The PI3K-related kinase (PIKK) SMG1 monitors the progression of metazoan nonsense-mediated mRNA decay (NMD) by phosphorylating the RNA helicase UPF1. SMG1 is a member of the phosphatidylinositol-3-kinase-related kinase (PIKK) family, which also includes the ATM, ATR, DNA-PKc, and mTOR kinases. Despite the confounding name reflecting a possible evolutionary origin with a lipid kinase, and in retrospect the ability of some PIKK family members to bind inositol-6-phosphate, all active PIKKs are Ser-Thr protein kinases. These large, multidomain enzymes share an overall similar architecture: a C-terminal catalytic module (comprising the so-called FAT, kinase, and FATC domains) and an N-terminal α-solenoid (that typically serves as a protein-protein interaction module). SMG8 and SMG9 form an unusual G-domain heterodimer.

In this manuscript, we reported a reconstruction of the SMG1-8-9 complex bound to an SMG1 inhibitor. We showed that this compound binds to the ATP-binding site within the kinase active site. While many of the SMG1 residues interacting with SMG1i are conserved within the PIKK family, two contact sites appear to be specific: SMG1 Pro2213 and Asp2339 contact the sulfonamide moiety of the inhibitor while Asn2356 forms hydrogen bonds with the phenyl urea/carbamide group. Superposition of the SMG1 active site in the SMG1i-bound structure with the active site of mTORΔN shows that the corresponding residues have diverged and would not be able to mediate analogous interactions with the SMG1i sulfonamide group (mTOR Thr2245 and Ser2342 at the positions of SMG1 Pro2213 and Asp2339) or with the urea group (mTOR Gly2359 at the position of SMG1 Asn2356). Taken together, these observations rationalize the specificity of SMG1i for SMG1 over mTORΔN that we observed in the in vitro assays. Superposition with other PIKKs suggests the presence of potentially similar discriminatory interactions: like mTOR, DNA-PK lacks a favorable interaction site for the SMG1i urea group (Gly3943 at the position of SMG1 Asn2356). In the case of ATR, the SMG1i sulfonamide site has diverged (Gly2385 at the position of SMG1 Pro2213) and residues in the N-lobe would result in a steric clash with the urea group of the inhibitor (Lys2329 and Asp2330 corresponding to SMG1 Leu2157 and Glu2158). Finally, mTOR, DNA-PK, and ATR active sites have a different relative orientation of the kinase N- and C-lobes as compared to SMG1, changing the overall chemical environment at the SMG1i-binding site. We conclude that subtle differences in the SMG1 structure underpin the specificity of the SMG1i inhibitor.

> ANTLVEDVNICLQACSSLHALSSSLPDDLLQRCVDVCRVQLVHSGTRIRQAFGKLLKSIPLDVVLSNNNHTEIQEISLALRSHMSKAPSNTFHPQDFSDVISFILYGNSHRTGKDNWLERLFYSCQRLDKRDQSTIPRNLLKTDAVLWQWAIWEAAQFTVLSKLRTPLGRAQDTFQTIEGIIRSLAAHTLNPDQDVSQWTTADNDEGHGNNQLRLVLLLQYLENLEKLMYNAYEGCANALTSPPKVIRTFFYTNRQTCQDWLTRIRLSIMRVGLLAGQPAVTVRHGFDLLTEMKTTSLSQGNELEVTIMMVVEALCELHCPEAIQGIAVWSSSIVGKNLLWINSVAQQAEGRFEKASVEYQEHLCAMTGVDCCISSFDKSVLTLANAGRNSASPKHSLNGESRKTVLSKPTDSSPEVINYLGNKACECYISIADWAAVQEWQNSIHDLKKSTSSTSLNLKADFNYIKSLSSFESGKFVECTEQLELLPGENINLLAGGSKEKINMKKLLPNMLSPDPRELQKSIEVQLLRSSVCLATALNPIEQDQKWQSITENVVKYLKQTSRIAIGPLRLSTLTVSQSLPVLSTLQLYCSSALENTVSNRLSTEDCLIPLFSEALRSCKQHDVRPWMQALRYTMYQNQLLEKIKEQTVPIRSHLMELGLTAAKFARKRGNVSLATRLLAQCSEVQLGKTTTAQDLVQHFKKLSTQGQVDEKWGPELDIEKTKLLYTAGQSTHAMEMLSSCAISFCKSVKAEYAVAKSILTLAKWIQAEWKEISGQLKQVYRAQHQQNFTGLSTLSKNILTLIELPSVNTMEEEYPRIESESTVHIGVGEPDFILGQLYHLSSVQAPEVAKSWAALASWAYRWGRKVVDNASXXXXXXXXXXXXXXXXXXXXXXXXXXXXXXXXXXXXXXXXXXXXXXXXXXXXXXXXXXXXXXXXXXXXXXXXXXXXXXXXXXXXXXXXEGVIKVWRKVVDRIFSLYKLSCSAYFTFLKLNAGQIPLDEDDPRLHLSHRVEQSTDDMIVMATLRLLRLLVKHAGELRQYLEHGLETTPTAPWRGIIPQLFSRLNHPEVYVRQSICNLLCRVAQDSPHLILYPAIVGTISLSSESQASGNKFSTAIPTLLGNIQGEELLVSECEGGSPPASQDSNKDEPKSGLNEDQAMMQDCYSKIVDKLSSANPTMVLQVQMLVAELRRVTVLWDELWLGVLLQQHMYVLXXXXXXXXXXXXXXXXXXXXXXXXXXXXXXXXXXXXXXXXXXXXXXXXXXXXXXXXPHEKWFQDNYGDAIENALEKLKXXXXXXXXXXXXXXXXXXXXXXXXXXXXXXXYILRLEEISPWLAAMTNTEIALPGEVSARDTVTIHSVGGTITILPTKTKPKKLLFLGSDGKSYPYLFKGLEDLHLDERIMQFLSIVNTMFATINRQETPRFHARHYSVTPLGTRSGLIQWVDGATPLFGLYKRWQQREAALQAQKAQDSYQTPQNPGIVPRPSELYYSKIGPALKTVGLSLDVSRRDWPLHVMKAVLEELMEATPPNLLAKELWSSCTTPDEWWRVTQSYARSTAVMSMVGYIIGLGDRHLDNVLIDMTTGEVVHIDYNVCFEKGKSLRVPEKVPFRMTQNIETALGVTGVEGVFRLSCEQVLHIMRRGRETLLTLLEAFVYDPLVDWTAGGEAGFAGAVYGGGGQQAESKQSKREMEREITRSLFSSRVAEIKVNWFKNRDEMLVVLPKLDGSLDEYLSLQEQLTDVEKLQGKLLEEIEFLEGAEGVDHPSHTLQHRYSEHTQLQTQQRAVQEAIQVKLNEFEQWITHYQAAFNNLEATQLASLLQEISTQMDLGPPSYVPATAFLQNAGQAHLISQCEQLEGEVGALLQQRRSVLRGCLEQLHHYATVALQYPKAIFQKHRIEQWKTWMEELICNTTVERCQELYRKYEMQYAPQPPPTVCQFITATEMTLQRYAADINSRLIRQVERLKQEAVTVPVCEDQLKEIERCIKVFLHENGEEGSLSLASVIISALCTLTRRNLMMEGAASSAGEQLVDLTSRDGAWFLEELCSMSGNVTCLVQLLKQCHLVPQDLDIPNPMEASETVHLANGVYTSLQELNSNFRQIIFPEALRCLMKGEYTLESMLHELDGLIEQTTDGVPLQTLVESLQAYLRNAAMGLEEETHAHYIDVARLLHAQYGELIQPRNGSVDETPKMSAGQMLLVAFDGMFAQVETAFSLLVEKLNKMEIPIAWRKIDIIREARSTQVNFFDDDNHRQVLEEIFFLKRLQTIKEFFRLCGTFSKTLSGSSSLEDQNTVNGPVQIVNVKTLFRNSCFSEDQMAKPIKAFTADFVRQLLIGLPNQALGLTLCSFISALGVDIIAQVEAKDFGAESKVSVDDLCKKAVEHNIQIGKFSQLVMNRATVLASSYDTAWKKHDLVRRLETSISSCKTSLQRVQLHIAMFQWQHEDLLINRPQAMSVTPPPRSAILTSMKKKLHTLSQIETSIATVQEKLAALESSIEQRLKWAGGANPALAPVLQDFEATIAERRNLVLKESQRASQVTFLCSNIIHFESLRTRTAEALNLDAALFELIKRCQQMCSFASQFNSSVSELELRLLQRVDTGLEHPIGSSEWLLSAHKQLTQDMSTQRAIQTEKEQQIETVCETIQNLVDNIKTVLTGHNRQLGDVKHLLKAMAKDEEAALADGEDVPYENSVRQFLGEYKSWQDNIQTVLFTLVQAMGQVRSQEHVEMLQEITPTLKELKTQSQSIYNNLVSFASPLVTDATNECSSPTSSATYQPSFAAAVRSNTGQKTQPDVMSQNARKLIQKNLATSADTPPSTVPGTGKSVACSPKKAVRDPKTGKAVQERNSYAVSVWKRVKAKLEGRDVDPNRRMSVAEQVDYVIKEATNLDNLAQLYEGWTAWV> TKVVEISPTTRLEGHSKLTLKVNDQGIVERGDWLSITPVRGIEKLAIGKTMEQVPKIASRVCGICPIAHTLASTEAMEASIGCEIPTDAKLLRIILHAANRIHSHALHNILILPDFYIPGTEKKFNLFANEQPARSVMARIVRIREIAQTIAAIAGGEAIHPSNPRIGGMYHNVSPRAKQKMADLAKECLVLVHEQMEFMLDVIRNMQNREFVEVGGKQIPLPKKLGYHNQGVMATAPMYGSSSLDDNPTWDFTRWKETRPWDWYMGEVTIDLEDPSYPIGGTTKVGTKANPQMESCTGVPTYDGQPVEVGPRARLATFKNFDEKGTFAQHIARQMEYPDCCYTILNCLDNLNTSGKVLADHIPQGDGSMGWAANEAPRGSNIHLARVKDGKVRWYDMLVPTTWNFPTCSRALTGAPWQIAEMVVRAYDPCVSCATH;> MIEDPYLGKYVTCVSARSTDKEILKKAQDGGIATALMVYALEEGFIDGTIVAGEGDKPWQPKPVVAMTREDILKARGTRYNISPQISWLKEATRSFGLDKVGVTGVCCQMQAVRKAQLYPINMRDVPGKVAFTVGLFCMENFSYKSLQSIVEDHANQSLGSVKKMEITKGKFWVYTERGNVATVPLKATHKYEQPGCHVCLDYVSNLADISTGSVGSPDGWSTVFIRTKVGNEIWSKAVADGMFETKPIEEVK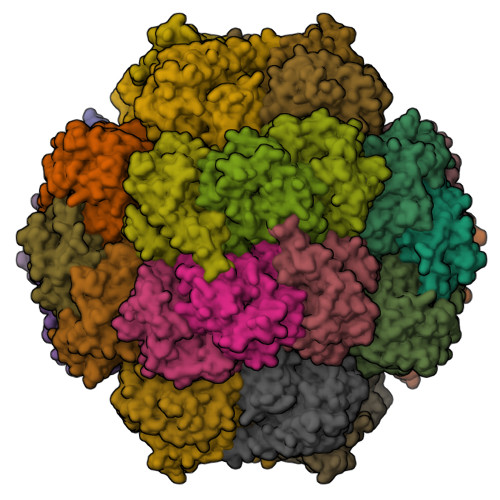PGLDLLRKLAKQKIDKNQKTVEERKTFGINKGLRNPYA;> TNKIKIGHVHMSGCTGCLVSLADNNLGLIKILDDYADLVYCLTLADVRHIPEMDVALVEGSVCLQDHESVEDIKETRKKSKIVVALGSCACYGNITRFSRGGQHNQPQHESYLPIGDLIDVDVYIPGCPPSPELIRNVAVMAYLLLEGNEEQKELAGKYLKPLMDLAKRGTSGCFCDLMYDVINQGLCMGCGTCAASCPVHAITLEFGKPQGERDLCIKCGSCYGACPRSFFNLDVISEFENISEIIAKALKD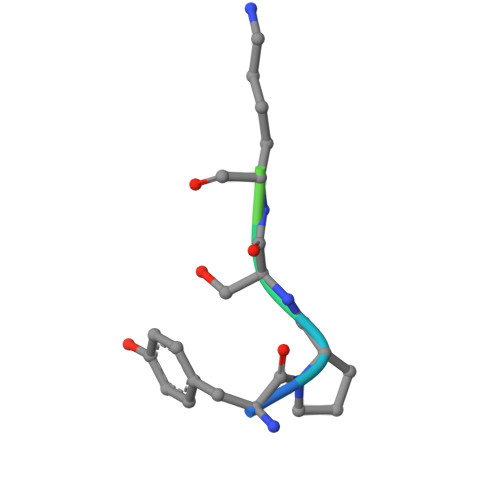> YPSKPDNPGE> MIQKVITVNGIEQNLFVDAEALLSDVLRQQLGLTGVKVGCEQGQCGACSVILDGKVVRACVTKMKRVADGAQITTIEGVGQPENLHPLQKAWVLHGGAQCGFCSPGFIVSAKGLLDTNADPSREDVRDWFQKHRNACRCTGYKPLVDAVMDAAAVINGKKPETDLEFKMPADGRIWGSKYPRPTAVAKVTGTLDYGADLGLKMPAGTLHLAMVQAKVSHANIKGIDTSEALTMPGVHSVITHKDVKGKNRITGLITFPTNKGDGWDRPILCDEKVFQYGDCIALVCADSEANARAAAEKVKVDLEELPAYMSGPAAAAEDAIEIHPGTPNVYFEQPIVKGEDTGPIFASADVTVEGDFYVGRQPHMPIEPDVAFAYMGDDGKCYIHSKSIGVHLHLYMIAPGVGLEPDQLVLVANPMGGTFGYKFSPTSEALVAVAAMATGRPVHLRYNYQQQQQYTGKRSPWEMNVKFAAKKDGTLLAMESDWLVDHGPYSEFGDLLTLRGAQFIGAGYNIPNIRGLGRTVATNHVWGSAFRGYGAPQSMFASECLMDMLAEKLGMDPLELRYKNAYRPGDTNPTGQEPEVFSLPDMIDQLRPKYQAALEKAQKESTATHKKGVGISIGVYGSGLDGPDASEAWAELNADGTITVHTAWEDHGQGADIGCVGTAHEALRPMGVAPEKIKFTWPNTATTPNSGPSGGSRQQVMTGNAIRVACENLLKACEKPGGGYYTYDELKAADKPTKITGNWTASGATHCDAVTGLGKPFVVYMYGVFMAEVTVDVATGQTTVDGMTLMADLGSLCNQLATDGQIY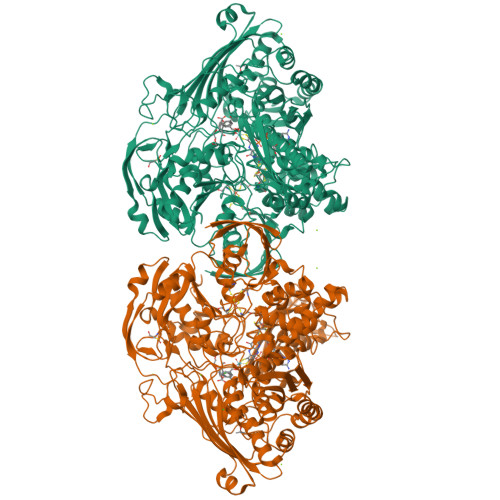GGLAQGIGLALSEDFEDIKKHATLVGAGFPFIKQIPDKLDIVYVNHPRPDGPFGASGVGELPLTSPHAAIINAIKSATGVRIYRLPAYPEKVLEALKA>MAAPDLLDPKSATHNTKPRLSFSSKPIVYNSGDDCESITTVMKWKTVLAIFLLV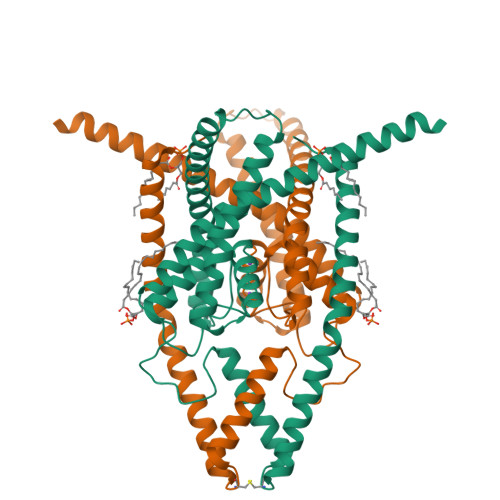VLYLIIGATVFKALEQPEEGLQKYRIIQEKIDFLSMHTCVQTSELEDLVKQVVLAIRAGVNPSGHPSQESSMWDLSSSFFFAGTVITTIGFGNVSPHTEGGRIFCIIYALLGIPLFGFLLAGVGDQLGTIFGKGIAKVEKMFVKWNVSQTKIRVTSTVLFILFGCLLFVALPALIFQHIEGWSALESIYFVVITLTTIGFGDFVAGGSEIEYLDYYKPIVWFWILVGLAYFAAVLSMIGDWLRVISKKTKEEVGEFRAHAAEWTANV[2x]>[2x]MTYNIILAKSALELIPEEIKNKIRKSRVY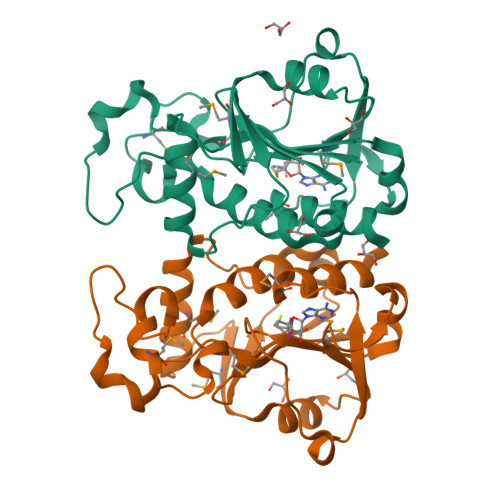KYDILDSNYHYKAMEKLKDKEMRGRPDIIHISLLNILDSPINHEKKLNIYIHTYDDKVLKINPETRLPRNYFRFLGVMEKVLKGERNHLIKMEEKTLEDLLNEINAKKIAIMTKTGKLTHPKLLKEYDTFIIGGFPYGKLKINKEKVFGDIKEISIYNKGLMAWTVCGIICYSLSF>[4x]PCPPTNAERLHEFHRAIGAATPERPTPPPPELLRLRQTLLDEASAEVRAEIDHLLARQAAGEALSAGDLAPLA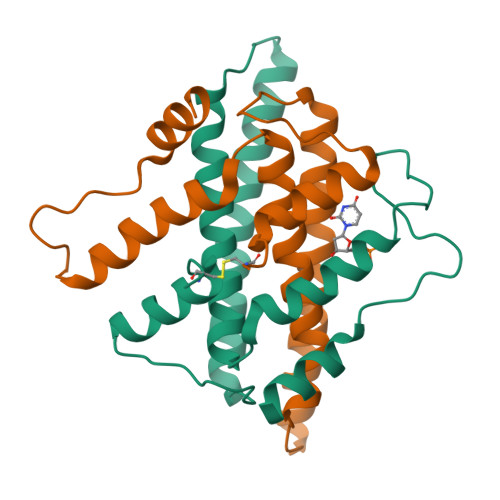HELADLLYVTYGALDQLGIDADAVFAEVHRANLSKASGPRRADGKQLKPEGWRPADVRGVIERLQHA> SVTIDHTTENAAPAQAPVSDRAWALFRALDGKGLVPDGYVEGWKKTFEEDFSPRRGAELVARAWTDPEFRQLLLTDGTAAVAQYGYLGPQGEYIVAVEDTPTLKNVIVCSLCSCTAWPILGLPPTWYKSFEYRARVVREPRKVLSEMGTEIASDIEIRVYDTTAETRYMVLPQRPAGTEGWSQEQLQEIVTKDCLIGVAIPQVPTV;> MDGVHDLAGVQGFGKVPHTVNADIGPTFHAEWEHLPYSLMFAGVAELGAFSVDEVRYVVERMEPRHYMMTPYYERYVIGVATLMVEKGILTQDELESLAG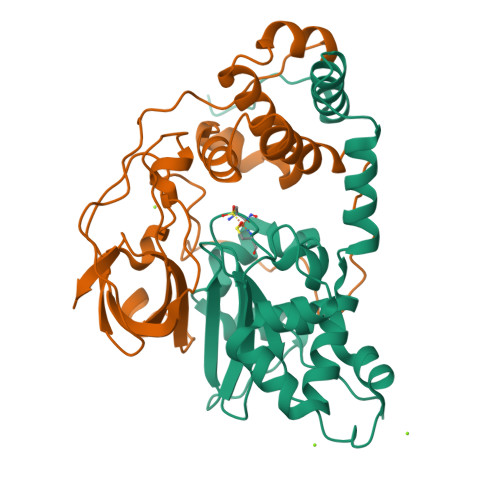GPFPLSRPSESEGRPAPVETTTFEVGQRVRVRDEYVPGHIRMPAYCRGRVGTISHRTTEKWPFPDAIGHGRNDAGEEPTYHVKFAAEELFGSDTDGGSVVVDLFEGYLEPAA>HHHHHHLESTSLYKKAGMATANGAVENGQPDRKPPALPRPIRNLEVKFTKIFINNEWHESKSGKKFATCNPSTREQICEVEEGDKPDVDKAVEAAQVAFQRGSPWRRLDALSRGRLLHQLADLVERDRATLAALETMDTGKPFLHAFFIDLEGCIRTLRYFAGWADKIQGKTIPTDDNVVCFTRHEPIGVCGAITPWNFPLLMLVWKLAPALCCGNTMVLKPAEQTPLTALYLGSLIKEAGFPPGVVNIVPGFGPTVGAAISSHPQINKIAFTGSTEVGKLVKEAASRSNLKRVTLELGGKNPCIVCADADLDLAVECAHQGVFFNQGQCCTAASRVFVEEQVYSEFVRRSVEYAKKRPVGDPFDVKTEQGPQIDQKQFDKILELIESGKKEGAKLECGGSAMEDKGLFIKPTVFSEVTDNMRIAKEEIFGPVQPILKFKSIEEVIKRANSTDYGLTAAVFTKNLDKALKLASALESGTVWINCYNALYAQAPFGGFKMSGNGRELGEYALAEYTEVKTVTIKLGDKNP[8x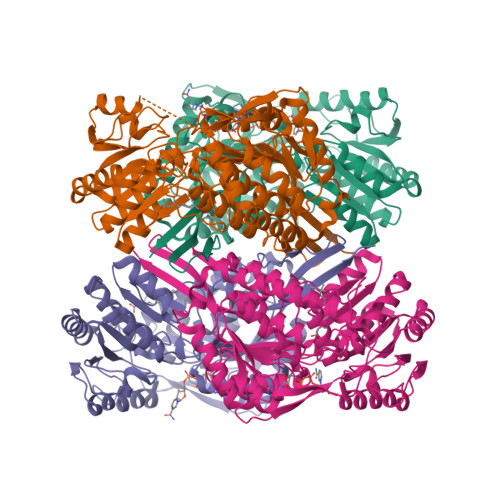]>MSLRSDLINALYDENQKYDVCGIISAEGKIYPLGSDTKVLSTIFELFSRPIINKIAEKHGYIVEEPKQQNHYPDFTLYKPSEPNKKIAIDIKTTYTNKENEKIKFTLGGYTSFIRNNTKNIVYPFDQYIAHWIIGYVYTRVATRKSSLKTYNINELNEIPKPYKGVKVFLQDKWVIAGDLAGSGNTTNIGSIHAHYKDFVEGKGIFDSEDEFLDYWRNYERTSQ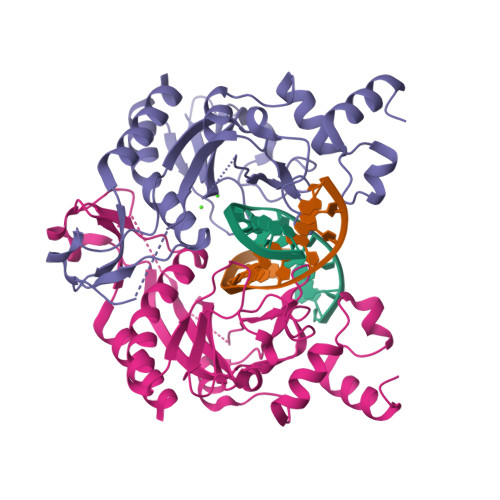LRNDKYNNISEYRNWIYRGRK[2x]methylglyoxal | C3 H4 O2 | 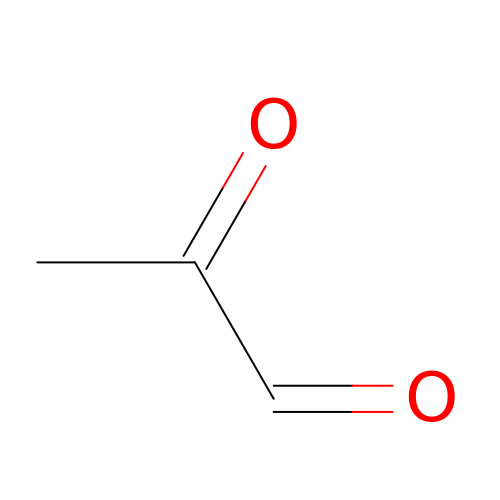AIJULSRZWUXGPQ-UHFFFAOYSA-N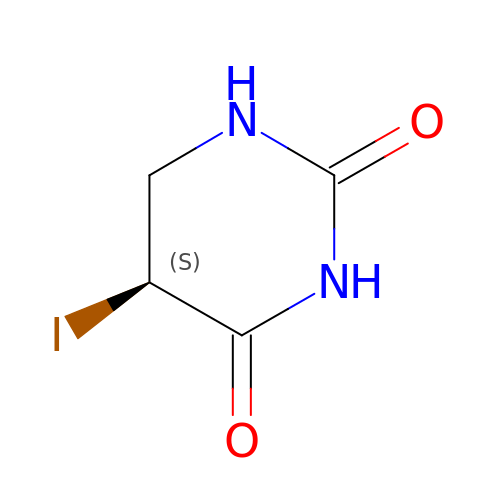(5S)-5-IODODIHYDRO-2,4(1H,3H)-PYRIMIDINEDIONE | C4 H5 I N2 O2 | YGKCTZPSAOUUMT-REOHCLBHSA-N N-{[5-AMINO-1-(5-O-PHOSPHONO-BETA-D-ARABINOFURANOSYL)-1H-IMIDAZOL-4-YL]CARBONYL}-L-ASPARTIC ACID | C13 H19 N4 O12 P | 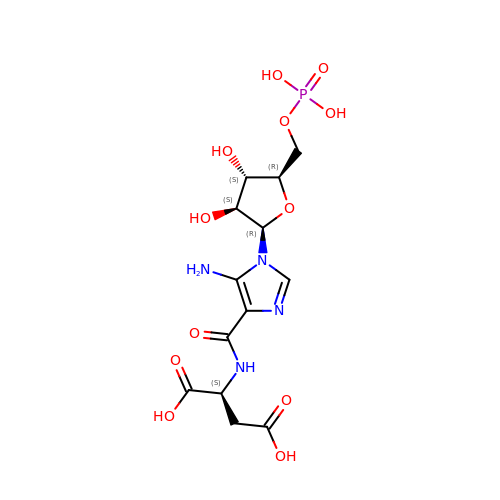NAQGHJTUZRHGAC-PSYSQGJASA-N> EIDALEFENDALEQKIAA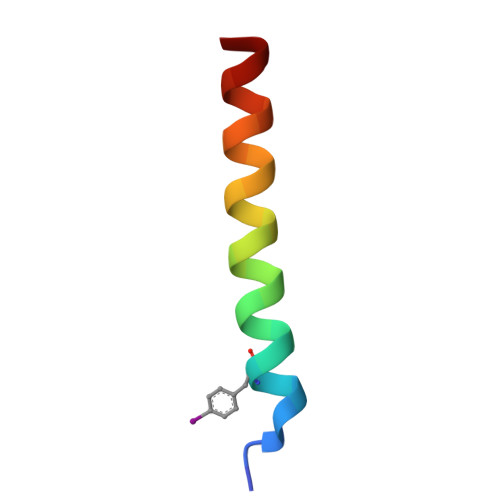LKQKIASLKQ> PGPVPPSTALRELIEELVNITQNQKAPLCNGSMVWSINLTTAGMYCAALESLINVSGCSAIEKTQRMLSGFCPHKVSAGQFSSLHVRDTKIEVAQFVKDLLLHLKKLFREGQFNRNFESIIICRDRT;> ADPFKVLQEPTCVSDYMSISTCEWKMNGPTQCSTELRLLYQLVFLLSEAHTCIPENNGGAGCVCHLLMDDVVSADQYTLDLWAGQQLLWKGSFKPSEHVKPRAPGNLTVHTQVSDTLLLTWSNPYPPDNYLY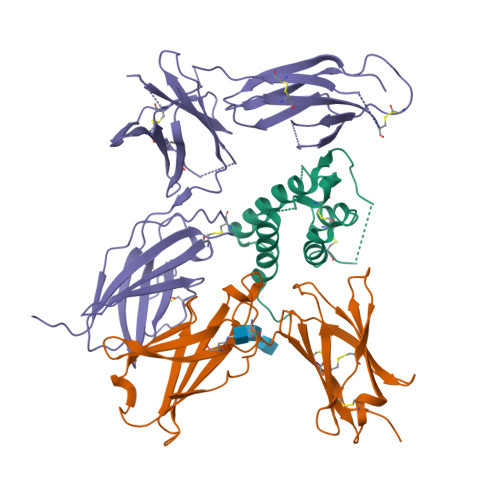NHLTYAVNIWSENDPADFRIYQVTYLEPSLRIAASTLKSGISYRARVRAWAQCYNTTWSEWSPSTKWHNSYRE;> TETQPPVTNLSVSVENLCTVIWTWNPPEGASSNCSLWYFSHFGDKQDKKIAPETRRSIEVPLNERICLQVGSQCSTNESEKPSILVEKCISPPEGDPESAVTELQCIWHNLSYMKCSWLPGRNTSPDTNYTLYYWHRSLEKIHQCENIFREGQYFGCSFDLTKVKDSSFEQHSVQIMVKDNAGKIKPSFNIVPLTSRVKPDPPHIKNLSFHNDDLYVQWENPQNFISRCLFYEVEVNNSQTETHNVFYVQEAKCENPEFERNVENTSCFMVPGVLPDTLNTVRIRVKTNKLCYEDDKLWSNWSQEMSIGKKRNS> SKGK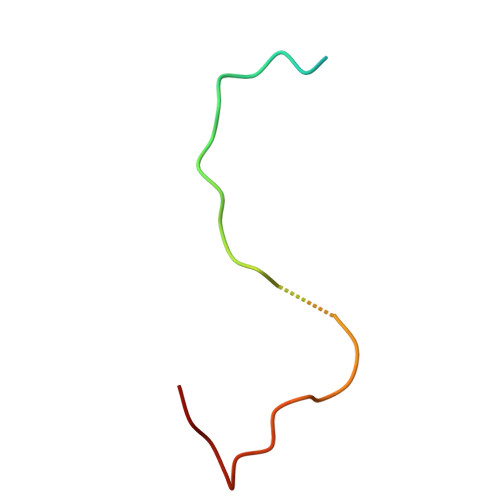KRSGARPGRPQPLRGTKGKRKGARLWYVGGQQF> CVTQLLKDTCFEGGDITTVFTPSAKYCQVVCTYHPRCLLFTFTAESPSEDPTRWFTCVLKDSVTETLPRVNRTAAISGYSFKQCSHQISACNKDIYVDLDMKGINYNSSVAKSAQECQERCTDDVHCHFFTYATRQFPSLEHRNICLLKHTQTGTPTRITKLDKVVSGFSLKSCALSNLACIRDIFPNTVFADSNIDSVMAPDAFVCGRICTHHPGC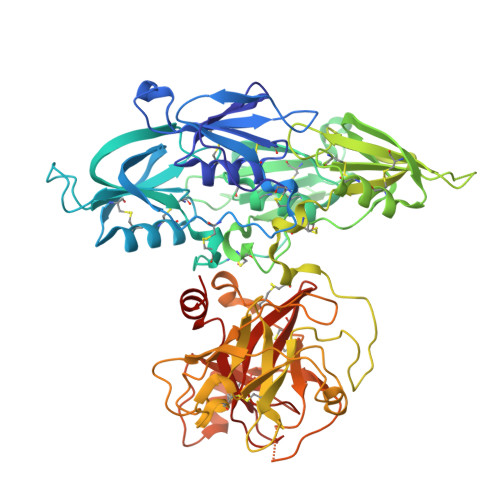LFFTFFSQEWPKESQRNLCLLKTSESGLPSTRIKKSKALSGFSLQSCRHSIPVFCHSSFYHDTDFLGEELDIVAAKSHEACQKLCTNAVRCQFFTYTPAQASCNEGKGKCYLKLSSNGSPTKILHGRGGISGYTLRLCKMDNECTTKIKPRIVGGTASVRGEWPWQVTLHTTSPTQRHLCGGSIIGNQWILTAAHCFYGVESPKILRVYSGILNQSEIKEDTSFFGVQEIIIHDQYKMAESGYDIALLKLETTVNYTDSQRPICLPSKGDRNVIYTDCWVTGWGYRKLRDKIQNTLQKAKIPLVTNEECQKRYRGHKITHKMICAGYREGGKDACKGDSGGPLSCKHNEVWHLVGITSWGEGCAQRERPGVYTNVVEYVDWILEKTQAV>[4x]GFMKGIYSALMVPYNEDGSINEKGLREIIRYNIDKMKVDGLYVGGSTGENFMISTEEKKRVFEIAIDEAKDSVNLIAQVGSINLNEAVELGKYVTKLGYKCLSAVTPFYYKFDFSEIKDYYETIVRETGNYMIIYSIPFLTGVNMSLSQFGELFENEKIIGVKFTAGDFYLLERVRKAFPDKLIFAGFDEMLLPATVLGVDGAIGSTYNINGIRAKQIFELAK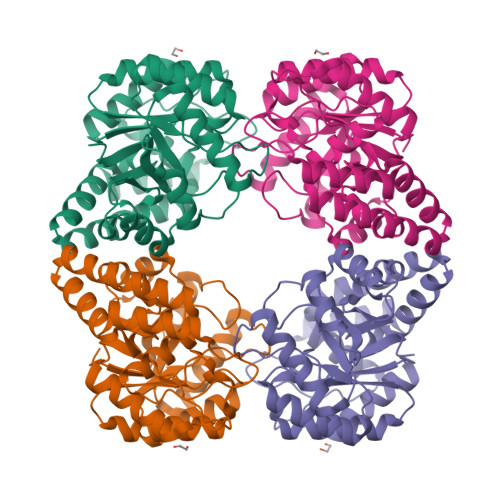NSKIDEALKIQHTTNDLIEGILSNGLYQTIKEILKLEGVDAGYCRKPMKKISQKQIEFAKELHKKFLK>MKFDPQKYRELAEKDFEAAWKAGKEILAERSPNELYPRVGFSFGKEHPLFATIQRLREAYLSIGFSEVVNPLIVEDVHVKKQFGREALAVLDRCFYLATLPKPNVGISAEKIRQIEAITKREVDSKPLQEIFHRYKKGEIDGDDLSYLIAEVLDVDDITAVKILDEVFPEFKELKPISSTLTLRSHMTTGWFITLSHIADKLPLPIKLFSIDRCFRREQGEDATRLYTYFSASCVLVDEELSVDDGKAVAEALLRQFGFENFRFRKDEKRSKYYIPDTQTEVFAFHPKLVGSSTKYSDGWIEIATFGIYSPTALAEYDIPYPVMNLGLGVERLAMILYGYDDVRKMVYPQIHGEIKLSDLDIAREIKVKE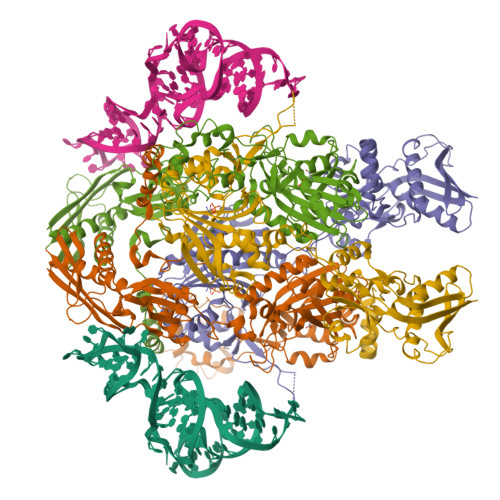VPQTAVGLKIAQSIVETAEKHASEPSPCSFLAFEGEMMGRNVRVYVVNENENTKLCGPAYANEVVVYKGDIYGIPKTKKWRSFFEEGVPTGIRYIDGFAYYAARKVEEAAMREQEEVKVKARIVENLSDINLYIHENVRRYILWKKGKIDVRGPLFVTVKAEIE[2x]6-methoxy-1,3-benzothiazol-2-amine | C8 H8 N2 O S | 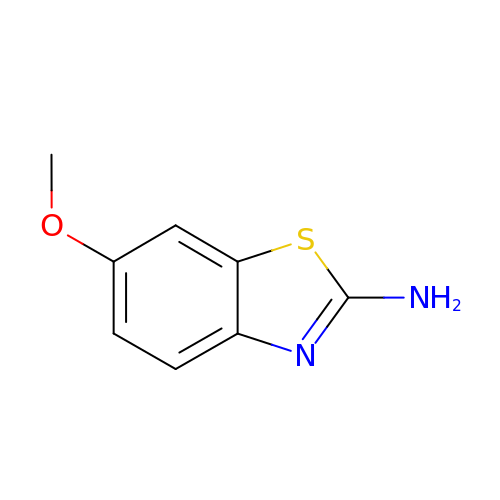KZHGPDSVHSDCMX-UHFFFAOYSA-N> MTEAQAIAKQLGGVKPDDEWLQAEIARLKGKSIVPLQQVKTLHDWLDGKRKARKSCRVVGESRTGKTVACD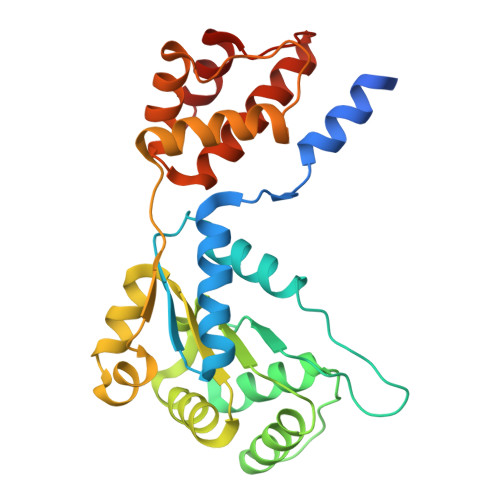AYRYRHKPQQEAGRPPTVPVVYIRPHQKCGPKDLFKKITEYLKYRVTKGTVSDFRDRTIEVLKGCGVEMLIIDEADRLKPETFADVRDIAEDLGIAVVLVGTDRLDAVIKRDEQVLERFRAHLRFGKLSGEDFKNTVEMWEQMVLKLPVSSNLKSKEMLRILTSATEGYIGRLDEILREAAIRSLSRGLKKIDKAVLQEVAKEYK>SMGFWEASSRGGGAFSGGEDASEGGAEEGAGGAGGSAGAGEGGVITALTPMTIPDVFPHLPLIAITRNPVFPRFIKIIEVKNKKLVELLRRKVRLAQPYVGVFLKRDDSNESDVVESLDEIYHTGTFAQIHEMQDLGDKLRMIVMGHRRVHISRQLEVEPEEPEAENKHKPRRKSKRGKKEAEDELSARHPAELAMEPTPELPAEVLMVEVENVVHEDFQVTEEVKALTAEIVKTIRDIIALNPLYRES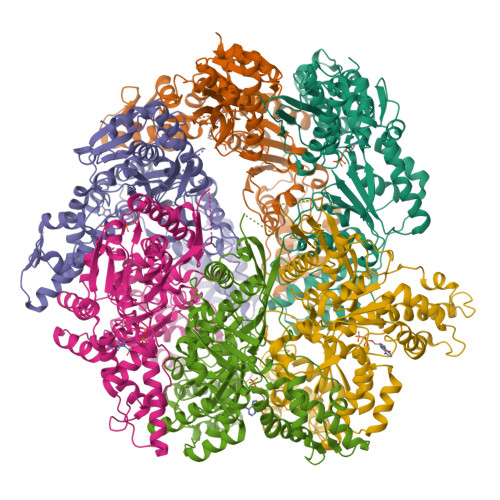VLQMMQAGQRVVDNPIYLSDMGAALTGAESHELQDVLEETNIPKRLYKALSLLKKEFELSKLQQRLGREVEEKIKQTHRKYLLQEQLKIIKKELGLEKDDKDAIEEKFRERLKELVVPKHVMDVVDEELSKLGLLDNHSSEFNVTRNYLDWLTSIPWGKYSNENLDLARAQAVLEEDHYGMEDVKKRILEFIAVSQLRGSTQGKILCFYGPPGVGKTSIARSIARALNREYFRFSVGGMTDVAEIKGHRWTYVGAMPGKIIQCLKKTKTENPLILIDEVDMIGRGYQGDPSSALLELLDPEQNANFLDHYLDVPVDLSKVLFICTANVTDTIPEPLRDRMEMINVSGYVAQEKLAIAERYLVPQARALCGLDESKAKLSSDVLTLLIKQYCRESGVRNLQKQVEKVLRKSAYKIVSGEAESVEVTPENLQDFVGKPVFTVERMYDVTPPGVVMGLAWTAMGGSTLFVETSLRRPQDKDAKGDKDGSLEVTGQLGEVMKESARIAYTFARAFLMQHAPANDYLVTSHIHLHVPEGATPKDGPSAGCTIVTALLSLAMGRPVRQNLAMTGEVSLTGKILPVGGIKEKTIAAKRAGVTCIVLPAENKKDFYDLAAFITEGLEVHFVEHYREIFDIAFPD[6x]N,N-dimethyl-L-valyl-L-leucyl-N-[(3S)-6-{(2S)-2-[(1H-indol-3-yl)methyl]-3-methoxy-5-oxo-2,5-dihydro-1H-pyrrol-1-yl}-6-oxo-1-phenylhexan-3-yl]-L-leucinamide 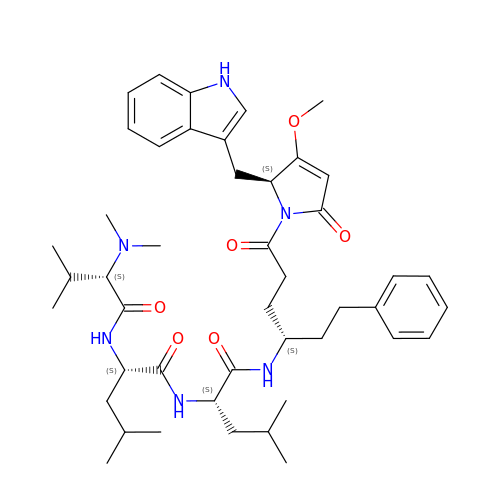| C45 H64 N6 O6 | YMHSWXIOFQGBAE-SDOACRIHSA-N> MMSKVKTRIYFCGGAGFRIGELFHGYHEDVCYIDTSVQNKHKHNTDDNTIIIEADTKLADQTARKRAIGMGKDRKAAAELISAHIPAIAHHFPAGDTNIVVYSMGGASGSTIGPSLVSHLQQQGEVVVSVVIGSYDSDISLRNSSGSLKTFEGVSSVSKVPMIINYHENVEGIPQSMVNQNILEVLNALVILFNQEHQSLDLMDITNWAHFHKHHDVPVQTVQLHVCFDRQEAQAILDPISIASLYTDPDRDVSISTVLTRTTGYADPEKYDFDQMHFVINGLSIEDIRKRLEERREMMNRAKANMRKRQSTLDVDDQATSSGLVFDHHHHHH

In this study, we looked at the protofilament contacts and filament structure formed by TubZ from Pseudomonas bacteriophage ΦKZ. We have solved the crystal structure of ΦKZ TubZ in the monomeric and polymeric forms, revealing structural changes in ΦKZ TubZ during polymerisation and showing that ΦKZ TubZ forms canonical tubulin/FtsZ subunit–subunit contacts and a functional tubulin/FtsZ active site. The crystal structures of ΦKZ TubZ revealed that it exhibits a tubulin/FtsZ protein family fold consisting of the canonical N-terminal GTP-binding domain, connected to the C-terminal GTPase activation domain through a conserved helix (H7). Tubulin/FtsZ family proteins frequently possess N- and C-terminal extensions to the conserved core, and although ΦKZ TubZ has no significant N-terminal extensions to the canonical fold, it possesses a flexible C-terminal helix (H11) similar to that found in Bacillus TubZs, C-ST TubZ,5 and 201Φ2-1 TubZ (PhuZ),6 which tails into a long extended coil at around residue 300 (of 327).

We solved the structure of crystals of ΦKZ TubZ to 2.0 Å (R/Rfree = 0.17/0.21); the asymmetric unit contained a single subunit of the protein in a monomeric state. The GTPase active site within the subunit was occupied by GDP, which was retained by ΦKZ TubZ through the purification process, and only the extreme N- and C-termini and a single region of surface loop T3 (residues 58–60) were not resolved within the electron density. The monomeric structure of ΦKZ TubZ exhibits several clear and interesting differences from those so far obtained for other tubulin/FtsZ family proteins. In terms of primary structure, there is a significant insertion within tubulin homology loop T3, which forms an α-helix instead of the conserved extended loop found in the majority of tubulin structures. Given the role of T3 in forming the subunit–subunit interface within a canonical protofilament, this would preclude formation of such a protofilament without significant rearrangement of the secondary structure. This is not the only such surface change, as the H10–S9 loop within the activation domain also lies in a conformation that would clash with an adjacent subunit and the partially disordered C-terminal tail prominent in previous TubZ structures lies across the subunit interface, blocking polymerisation. Combining structural information from both homologues, we propose that Pseudomonas TubZs may occupy a different conformation as a free monomer, surface loops being incorrectly ordered and the C-terminal helix and tail extending flexibly in solution as found in the monomeric ΦKZ structure.> EAQKQYWVCNSSDASISYTYCDKMQYPISINVNPCIELKGSKGLLHIFYIPRRDLKQLYFNLYITVNTMNLPKRKEVICRGSDDDYSFCRALKGE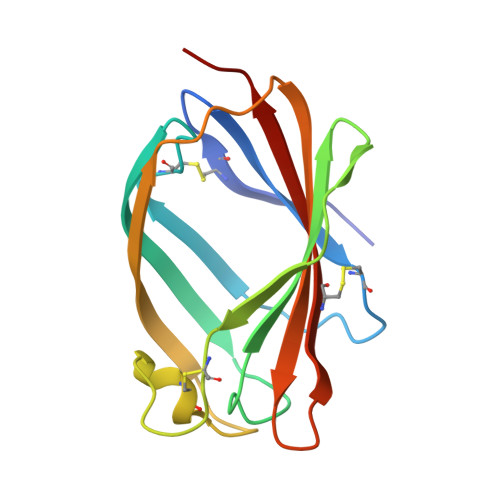TVNTTISFSFKGIKFSKGKYKCVVEAISGSPEEMLFCLEFVILHQPNSN The genomes of Bacteroidales contain genes encoding glycan-degrading apparatuses that typically co-localize in discrete clusters known as polysaccharide utilization loci (PULs). B. thetaiotaomicron contains almost 300 different GHs belonging to 60 different GH families, and secretes at least six mannosyl-glycoprotein endo-β-N-acetylglucosaminidases (ENGases, endoglycosidase hereafter) that hydrolyze the chitobiose core of asparagine-linked, or N-linked, glycans (EC 3.2.1.96). Here, we discover an ENGase from the GH18 family in B. thetaiotaomicron, BT1285, encoded in a distinct PUL with its own repertoire of proteins for catabolism of the same HM N-glycan substrate as that of BT3987. Altogether, our data suggest that human gut microbes employ evolutionary strategies to express distinct ENGases in order to optimally metabolize the same N-glycan substrate in the gastroinstestinal tract.

To better understand the molecular mechanism by which BT1285 specifically hydrolyzes N-glycans, we solved the crystal structure of a catalytically inactive variant of BT1285 (BT1285D161A-E163A; hereafter BT1285i) in complex with the Man9GlcNAc2 substrate at 1.9 Å resolution. We found one molecule of the Man9GlcNAc2 substrate unambiguously positioned in the active site of the enzyme flanked by the following connecting regions: β1–α1 (loop 1; residues 52–57), β2–α2 (beta hairpin; residues 78-94), β4–α3 (loop 2; residues 123–135), β5–α4 (loop 3; residues 161-178), β6–β7 (loop 4; residues 199–204), β7– β8 (loop 5; residues 218–240), β8–α5 (loop 6; residues 243-250), β9–α6 (loop 7; residues 272–282). We observed no substantial conformational changes in the protein backbone for the unliganded and glycan-bound forms of BT1285 (r.m.s.d. of 0.4 Å for 271 residues). For example, Man (−5) forms hydrogen bonds with residues E166 and R169 in BT1285 while it is exposed to solvent in BT3987, and Man (−9) is exposed to the solvent in BT1285, but it is in close contact with residue N403 in BT3987, These observations are consistent with the degrees of flexibility displayed by Mannoses within the crystal structures of both ENGases bound to HM-N-glycan, as evidenced by the B-factor values. To further investigate how BT1285 specifically recognizes HM substrates at the molecular level and how it compares to other HM-processing ENGases such as BT3987, we performed an alanine scanning mutagenesis analysis of residues that decorate the β-barrel core of the enzyme and contact the Man9GlcNAc2 N-linked glycan substrate. E52A from loop 1, H126A from loop 2, and E166 from loop3 drastically reduced the hydrolytic activity against IgG of the enzyme (at 37 °C, pH 7.4). Simultaneous mutation of two non-catalytic residues, Glu52 and His126, both of which engage the N-glycan core, completely abolished BT1285 hydrolytic activity, indicating that together these two residues are essential for HM substrate recognition.

>MPVNQSDNNQSEVVTRSATGIKNIVYIEVNDINPLNAGSYIMDDAPFFDYVILFAANIRGVGSDATLYNNPNVQYILDHKDTLIKPLQDKGIKVLLGLLGDHTGLGFANMNSAQTEQFATAVANAVSQYGLDGVDFADAWAEYGRNGYPSGSTGSFSNLITALHNKMPGKTITVFNYGYTSELTGVNSYIDYGIYAFFNSPSWSTGFGMPNSKFAPYTINLNSAPSAASAQLYSGQVASKGYGAIGYYDLRANNIVSVLNGVAKGAFKSTCTYDGNSYPKNY[2x]>[4x]MEAKTMKDMQKEVDAYIGQFK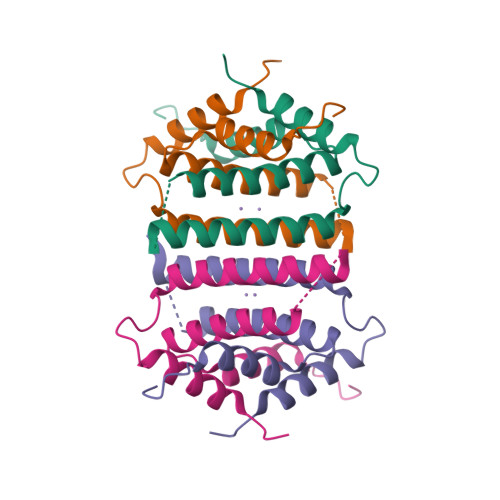EGYFSPLAMMARLTEEMGELAREVNHYYGEKPKKTTEKERSIEEELGDVLFVMICMANSLNIDLETAHNIVMNKFNTRDKDR>[4x]MAVTQSPRNKVAVTGGKVTLSCNQTNNHNNMYWYRQDTGHGLRLIHYSYGAG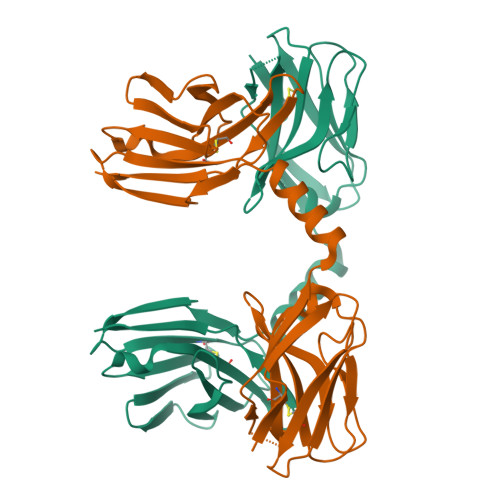STEKGDIPDGYKASRPSQENFSLILELATPSQTSVYFCASGDLGQTNERLFFGHGTKLSVLGSADDAKKDAAKKDGQVRQSPQSLTVWEGETAILNCSYENSAFDYFPWYQQFPGEGPALLISILSVSDKKEDGRFTIFFNKREKKLSLHIADSQPGDSATYFCAAIDTNAYKVIFGKGTHLHVLP(4S)-3-{[4-(4-cyano-2-methylphenyl)piperazin-1-yl]sulfonyl}-N-hydroxy-1,3-thiazolidine-4-carboxamide | C16 H21 N5 O4 S2 | 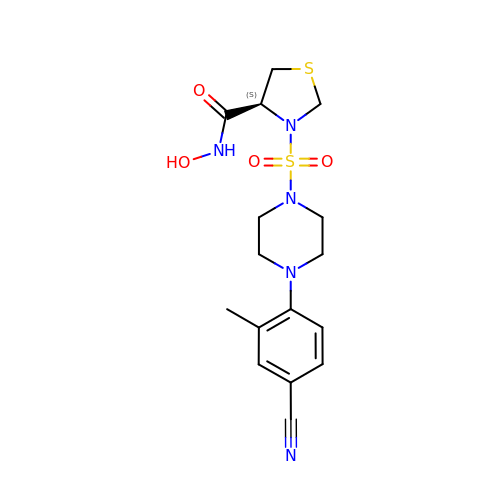UGVOWFLXYXPRQV-OAHLLOKOSA-N> MAEHGESSEDRISEIDYEFLPELSALLGVDAFQVAKSQEEEEHKERMKMKKGFNSQMRSEAKRLKTFETYDTFRSWTPQEMAAAGFYHTGVKLGVQCFCCSLILFGNSLRKLPIERHKKLRPECEFLQGKDVGNIGKYDIRVKSPEKMLRGGKARYHEEEARLESFEDWPFYAHGTSPRVLSAAGFVFTGKRDTVQCFSCGGSLGNWEEGDDPWKEHAKWFPKCEFLQSKKSSEEIAQYIQSYEGFVHVTGEHFVKSWVRRELPMVSAYCNDSVFANEELRMDMFKDWPQESPVGVEALVRAGFFYTGKKDIVRCFSCGGCLEKWAEGDDPMEDHIKFFPECVFLQTLKSSAEVIPTLQSQYALPEATETTRESNHGDAAAVHSTVVDLGRSEAQWFQEARSLSEQLRDNYTKATFRHMNLPEVC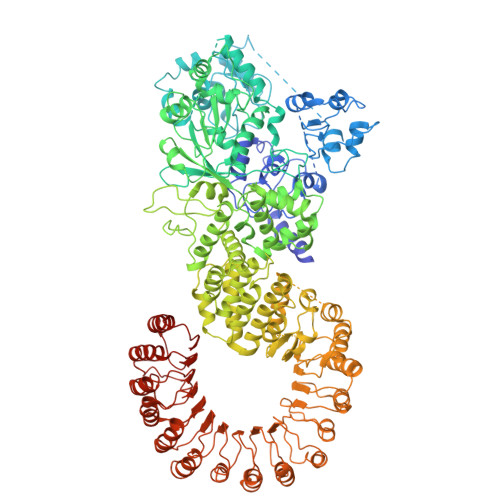SSLGTDHLLSCDVSIISKHISQPVQEALTIPEVFSNLNSVMCVEGETGSGKTTFLKRIAFLWASGCCPLLYRFQLVFYLSLSSITPDQGLANIICAQLLGAGGCISEVCLSSSIQQLQHQVLFLLDDYSGLASLPQALHTLITKNYLSRTCLLIAVHTNRVRDIRLYLGTSLEIQEFPFYNTVSVLRKFFSHDIICVEKLIIYFIDNKDLQGVYKTPLFVAAVCTDWIQNASAQDKFQDVTLFQSYMQYLSLKYKATAEPLQATVSSCGQLALTGLFSSCFEFNSDDLAEAGVDEDEKLTTLLMSKFTAQRLRPVYRFLGPLFQEFLAAVRLTELLSSDRQEDQDLGLYYLRQIDSPLKAINSFNIFLYYVSSHSSSKAAPTVVSHLLQLVDEKESLENMSENEDYMKLHPQTFLWFQFVRGLWLVSPESSSSFVSEHLLRLALIFAYESNTVAECSPFILQFLRGKTLALRVLNLQYFRDHPESLLLLRSLKVSINGNKMSSYVDYSFKTYFENLQPPAIDEEYTSAFEHISEWRRNFAQDEEIIKNYENIRPRALPDISEGYWKLSPKPCKIPKLEVQVNNTDAADQALLQVLMEVFSASQSIEFRLFNSSGFLESICPALELSKASVTKCSMSRLELSRAEQELLLTLPALQSLEVSETNQLPEQLFHNLHKFLGLKELCVRLDGKPDVLSVLPGEFPNLHHMEKLSIRTSTESDLSKLVKFIQNFPNLHVFHLKCDFLSNCESLMAVLASCKKLREIEFSGRCFEAMTFVNILPNFVSLKILNLKDQQFPDKETSEKFAQALGSLRNLEELLVPTGDGIHQVAKLIVRQCLQLPCLRVLTFHDILDDDSVIEIARAATSGGFQKLENLDISMNHKITEEGYRNFFQALDNLPNLQELNICRNIPGRIQVQATTVKALGQCVSRLPSLIRLHMLSWLLDEEDMKVINDVKERHPQSKRLIIFWKLIVPFSPVILE> MSILVNKNTKVIVQGFTGKEATFHAEQCMAYGTNIVGGITPHKGGQTHLGKPVFDTVADAVKATKADVSLIFVPAFAVGDSVIEAADAGIKLAVVITEHTPVKDMMFAKQYANKKGMKIIGPNCPGIITSEECKLGIMPGFIFKKGCVGLISKSGTLTYEAANQVVQGGYGISTAVGIGGDPIIGL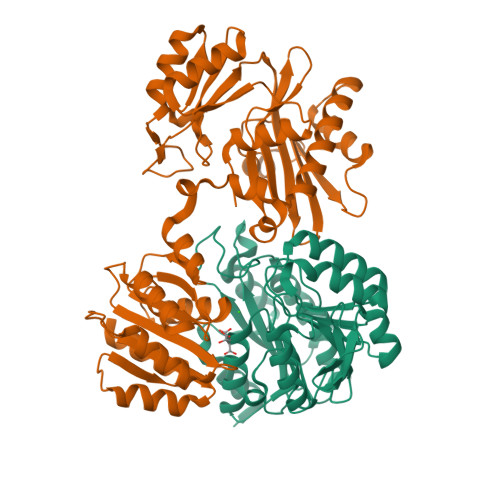AYKELLSEFQKDDETKAIVMIGEIGGSLEVEAAKFIKENISKPVVAFIAGATAPKGKRMGHAGAIVGSADESAAAKKEALKSYGIHVVDSPALIGEEIQKILGENLYFQ;> MNIHEYQAKAIFVDNGIPTLKGKVAFSVDEAVANAKELGGSVWAVKAQIHAGGRGLGGGVKIAKNLDEVKDYASKILGMNLVTHQTGPEGKLVQKLYIESGANIVKEYYLAILFNRMAEQITIIASSEGGMDIEKVAKESPEKIAKVGIDPQIGFKMFHGLEVARVLGLDKDEGKKLISMIAKLYKLYMDKDMNMLEINPLIKTAEGDFYALDAKCSFDDSALYRHPEIAELRDTTEENPAEREAAEFGLSYVKLDGDVACMVNGAGLAMATMDIINYSGAKPANFLDVGGGASPETVAKAFEIILRDKNVKVIFINIFGGIVRCDRIANGILEATKNVEVNIPIVVRLDGTNAAEAKTILDNSNLKNIKAATNLKNGAELVKSLVG>GHMTKLALFVRLEAKPGQEAALADFLASALPLANAESGTTAWFALKFGPSTFGVFDAFADEAGR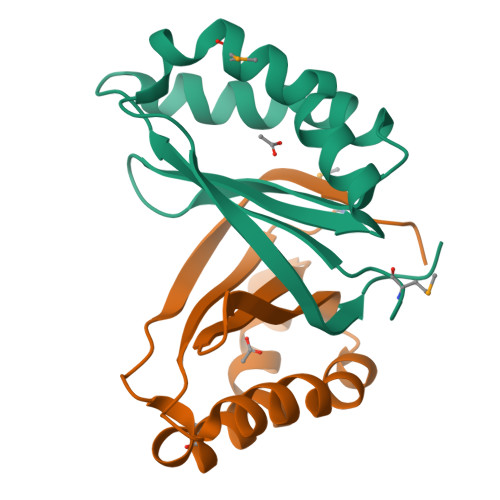QAHLNGQIAAALMANAATLLSSPPNIEKVELLAAKLPAGS[4x]The Nucleosome Remodelling and Deacetylase (NuRD) complex is a multi-protein chromatin modifying machine that plays an essential role in cell lineage commitment and DNA damage repair. The complex controls expression of genes through two distinct activities: removal of acetyl groups from chromatin through the action of a histone deacetylase enzyme and remodelling of nucleosomes through an ATP-dependent helicase. The deacetylase module from the NuRD complex contains three protein domains that control the recruitment of chromatin to the deacetylase enzyme, HDAC1/2. Using biochemical approaches and cryo-electron microscopy, we have determined how three chromatin-binding domains (MTA1-BAH, MBD2/3 and RBBP4/7) are assembled in relation to the core complex so as to facilitate interaction of the complex with the genome.

To understand the relationship between the BAH domain and the HDAC catalytic site, we prepared a complex containing an extended construct of MTA1 including the BAH, ELM2, SANT and GATA zinc finger (ZnF) domains (residues 1–453) together with HDAC1 and MBD2. CryoEM data were collected and a map was calculated to 4.5 Å based on 94 041 particles. A direct comparison of this map with that of the MTA1(ELM2-SANT):HDAC1:MBD2 complex shows that the central portion of the map is higher resolution than the first map and that the envelope of the complex extended, with additional density at either end of the HDAC1:MTA1 dimer. This part of the map has a distinctive, relatively narrow volume suggesting a compact but elongated domain which fits well with the known architecture of BAH domains. As would be expected, the position of the modelled BAH domain is such that the carboxy-terminus is close to the amino-terminal residue of the ELM2 domain. Although the GATA-like zinc-finger was included in this MTA1 construct, it was not possible to assign density for this in the map, and is speculatively positioned in our schematics. Importantly, we were also able to fit the BAH domains of MTA1 into the cryoEM map - even though this part of the map is comparatively less-well defined, likely due to some local motion of the BAH domains. We observe a striking arrangement of the BAH domains suggesting a potential mechanism for binding to di-nucleosomes. Certainly, the structure is compatible with two nucleosomes binding without clashes. Strikingly, the nucleosome would be positioned on the ‘top’ of the structure which would bring the histone tails into close proximity to the HDAC active site.

>[2x]MAANMYRVGDYVYFENSSSNPYLIRRIEELNKTANGNVEAKVVCFYRRRDISSTLIALADKHATLSVCYKAGPGADNGEEGEIEEEMENPEMVDLPEKLKHQLRHRELFLSRQLESLPATHIRGKCSVTLLNETESLKSYLEREDFFFYSLVYDPQQKTLLADKGEIRVGNRYQADITDLLKEGEEDGRDQSRLETQVWEAHNPLTDKQIDQFLVVARSVGTFARALDCSSSVRQPSLHMSAAAASRDITLFHAMDTLHKNIYDISKAISALVPQGGPVLCRDEMEEWSASEANLFEEALEKYGKDFTDIQQDFLPWKSLTSIIEYYYMWKTTDRYVQQKRLKAAEAESKLKQVYIPNYNKPNPNQISVNNVKAGVVNGTGAPGQSPGAGRACESCYTTQSYQWYSWGPPNMQCRLCASCWTYWKKYGGLKMPTRLDGERPGPNRSNMSPHGLPARSSGSPKFAMKTRQAFYLHTTKLTRIARRLCREILRPWHAARHPYLPINSAAIKAECTARLPEASQSPLVLKQAVRKPLEAVLRYLETHPRPPKPDPVKSVSSVLSSLTPAKVAPVINNGSPTILGKRSYEQHNGVDGNMKKRLLMPSRGLANHGQARHMGPSRNLLLNGKSYPTKVRLIRGGSLPPVKRRRMNWIDAPDDVFYMATEETRKIRKLLSSSETKRAARRPYKPIALRQSQALPPRPPPPAPVNDEPIVIED;>[2x]MAQTQGTRRKVCYYYDGDVGNYYYGQGHPMKPHRIRMTHNLLLNYGLYRKMEIYRPHKANAEEMTKYHSDDYIKFLRSIRPDNMSEYSKQMQRFNVGEDCPVFDGLFEFCQLSTGGSVASAVKLNKQQTDIAVNWAGGLHHAKKSEASGFCYVNDIVLAILELLKYHQRVLYIDIDIHHGDGVEEAFYTTDRVMTVSFHKYGEYFPGTGDLRDIGAGKGKYYAVNYPLRDGIDDESYEAIFKPVMSKVMEMFQPSAVVLQCGSDSLSGDRLGCFNLTIKGHAKCVEFVKSFNLPMLMLGGGGYTIRNVARCWTYETAVALDTEIPNELPYNDYFEYFGPDFKLHISPSNMTNQNTNEYLEKIKQRLFENLRMLPHAPGVQMQAIPEDAIPEESGDEDEDDPDKRISICSSDKRIACEEEFSDSEEEGEGGRKNSSNFKKAKRVKTEDEKEKDPEEKKEVTEEEKTKEEKPEAKGVKEEVKLA;> MRAHPGGGRCCPEQEEGESAAGGSGAGGDSAIEQGGQGSALAPSPVSGVRREGARGGGRGRGRWKQAGRGGGVCGRGRGRGRGRGRGRGRGRGRGRPPSGGSGLGGDGGGCGGGGSGGGGAPRREPVPFPSGSAGPGPRGPRATESGKRMDCPALPPGWKKEEVIRKSGLSAGKSDVYYFSPSGKKFRSKPQLARYLGNTVDLSSFDFRTGKMMPSKLQKNKQRLRNDPLNQNKGKPDLNTTLPIRQTASIFKQPVTKVTNHPSNKVKSDPQRMNEQPRQLFWEKRLQGLSASDVTEQIIKTMELPKGLQGVGPGSNDETLLSAVASALHTSSAPITGQVSAAVEKNPAVWLNTSQPLCKAFIVTDEDIRKQEERVQQVRKKLEEALMADILSRAADTEEMDIEMDSGDEA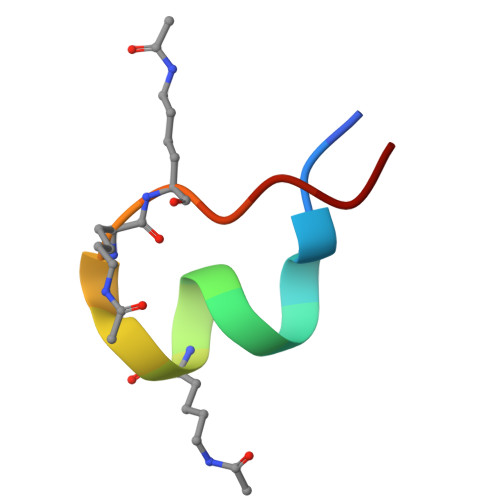> WYDVFLTRKYGKKKVAC> MAASGEARRVLVYGGRGALGSRCVQAFRARNWWVASIDVVENEEASASVIVKMTDSFTEQADQVTAEVGKLLGDQKVDAILCVA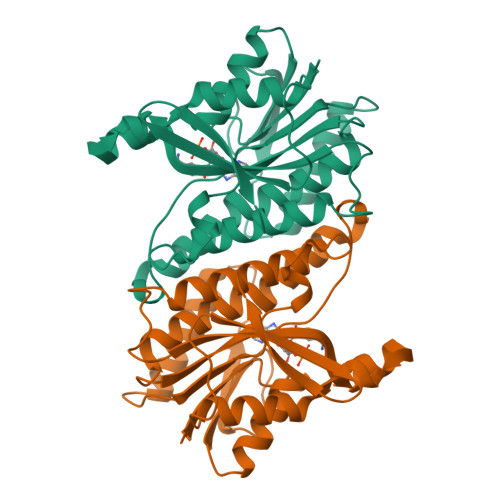GGWAGGNAKSKSLFKNCDLMWKQSIWTSTISSHLATKHLKEGGLLTLAGAKAALDGTPGMIGYGMAKGAVHQLCQSLAGKNSGMPSGAAAIAVLPVTLDTPMNRKSMPEADFSSWTPLEFLVETFHDWITGNKRPNSGSLIQVVTTDGKTELTPAYF>[2x]MENTENSVDSKSIKNLEPKIIHGSESMDSGISLDNSYKMDYPEMGLCIIINNKNFHKSTGMTSRSGTDVDAANLRETFRNLKYEVRNK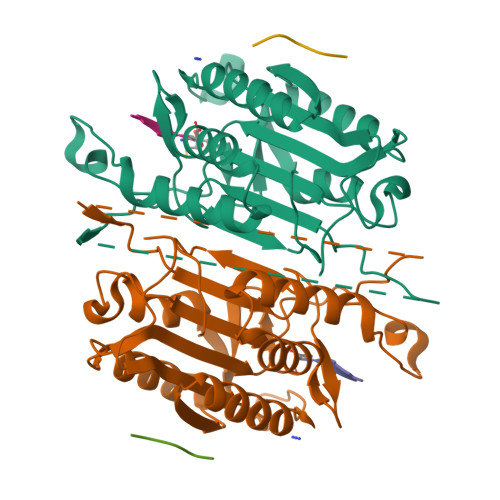NDLTREEIVELMRDVSKEDHSKRSSFVCVLLSHGEEGIIFGTNGPVDLKKITNFFRGDRCRSLTGKPKLFIIQACRGTELDCGIETDSGVDDDMACHKIPVEADFLFAYSTAPGYYSWRNSKDGSWFIQSLCAMLKQYADKLEFMHILTRVNRKVATEFESFSFDATFHAKKQIPCIHSMLTKELYFYH;>[2x]VDDDM>[2x]MHHHHHHHHHHSGDEVDAGSGQVDAGTMGTQKVTPALIFAITVATIGSFQFGYNTGVINAPEKIIKEFITKTLTDKGNAPPSEVLLTSLWSLSVAIFSVGGMIGSFSVGLFVNRFGRRNSMLIVNLLAVTGGCFMGLCKVAKSVEMLILGRLVIGLFCGLCTGFVPMYIGEISPTALRGAFGTLNQLGIVVGILVAQIFGLEFILGSEELWPLLLGFTILPAILQSAALPFCPESPRFLLINRKEEENAKQILQRLWGTQDVSQDIQEMKDESARMSQEKQVTVLELFRVSSYRQPIIISIVLQLSQQLSGINAVFYYSTGIFKDAGVQEPIYATIGAGVVNTIFTVVSLFLVERAGRRTLHMIGLGGMAFCSTLMTVSLLLKDNYNGMSFVCIGAILVFVAFFEIGPGPIPWFIVAELFSQGPRPAAMAVAGCSNWTSNFLVGLLFPSAAHYLGAYVFIIFTGFLITFLAFTFFKVPETRGRTFEDITRAFEGQAHGADRSGKDGVMEMNSIEPAKETTTNV

The major facilitator superfamily (MFS) glucose transporters (GLUTs), encoded by the SLC2 genes, mediate the transmembrane movement of various hexoses and derivatives in different tissues. The two domains, which exhibit a 2-fold pseudosymmetry around an axis that is perpendicular to the membrane plane, enclose a central cavity for substrate accommodation. Exposure of the substrate-binding site to either side of the membrane is achieved through rocker-switch rotation of the two domains as well as local conformational changes exemplified by the bending of TM722. The ligands that specifically bind to the outward- or inward-facing conformers of a transporter, wherein the substrate binding pocket is accessible to the extracellular or intracellular milieu, respectively, are defined as the exofacial or endofacial inhibitors.

To elucidate the mode of action (MOA) of SA47, we determined the crystal structure of SA47-bound WT GLUT3 (GLUT3-SA47) complex at 2.3 Å resolution. SA47 is unambiguously resolved in the central cavity, which opens to the extracellular side, consistent with the predicted outward-open conformation. Scrutiny of the electron density of SA47 reveals two conformers with regard to its pyrazoloaryl tail. The tail stretches towards the extracellular side in Conformer 1 and bends to be parallel with the membrane plane in Conformer 2. The piperazine moiety and the pyrazolopyrimidine core of SA47 partially overlay with the extracellular half of the glucose molecule. The aryl head stands aside the 3-hydroxy group of glucose, and the pyrazoloaryl tail projects to the extracellular side along the open tunnel. The comparison unambiguously shows the inhibitory mechanism of SA47 to be blocking substrate access to the central binding site. The structural shifts result in the displacement of the extracellular gating residue Tyr290, completing the transition from outward-occluded to outward-open. SA47 is coordinated by GLUT3 through extensive interactions, including hydrogen bonds (H-bonds), π stacking, and van der Waals contacts. The pyrazolopyrimidine moiety is stably bound via polar interactions with Gln159 on TM5, Asn315 on TM8, and Glu378 on TM8 and π-π stacking with Phe377 (bottom). While the benzyl group of the pyrazoloaryl tail forms a π-π stacking with Phe289 on TM7b, the two conformers of the aryl tail are coordinated differently by GLUT3 residues.>GSNEKIRSQSVLNTLETFFIKENHYDMQREESSIVNACLRYLGYSKSMCHEKMPIFMDIAFIEYCFNLSLDPSSFQNLPITQTQPDSQQILWEYSLISNALERLENIELERQNCMREDGLVKYTNELLLNKETLNNEALKLYSCAKAGICRWMAFHFLEQEPIDHINFTKFLQDWGSHNEKEMEALQRLSKHKIRKRLIYVSQHKKKMPWSKFNSVLSRYIQCTKLQLEVFCDYDFKQREIVKMLTSN[2x];>ACEMCRLGLP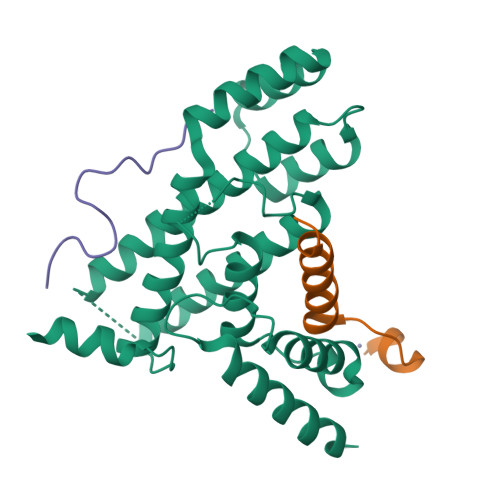HGSFFELLRDWKKIEEFRNKS[2x];>NSDNIFVKPGEDLEIPL[2x]> PGSMQDLTAQVTSDLLHFPEVTIEALGEDEITLESVLRGKFAAGKNGLACLACGPQLEVVNSLTGERLSAYRFSGVNEQPPVVLAVKEFSWHKRTGLLIGLEEADGSVLCLYDLGISRVVKAVVLPGRVTAIEPIINHGGASASTQHLHPSLRWLFGVAAVVTDVGQILLIDLCLDDLSCSQNEVEASDLEVITGIPAEVPHIRERVMREGRHLCFQLVSPLGVAISTLSYINRTNQLAVGFSDGYLALWNMKSMKREYYTQLEGGRVPVHAVAFQEPENDPRNCCYLWAVQSTQDSEGDVLSLHLLQLAFGDRKCLASGQILYEGLEYCEERYTLDLAGGTFPLRGQTSNTKLLGCQSIERFPSHGDREESMREALSPDTSVSVFTWQVNIYGQGKPSVYLGLFDINRWYHAQMPDSLRSGESLHNCSYFALWSLDSVVSRTSPHHILDIL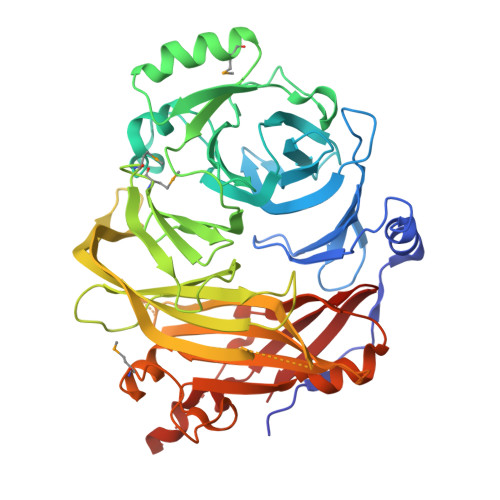VHERSLNRGVPPSYPPPEQFFNPSTFNFDATCLLDSGVIHVTCAG> IE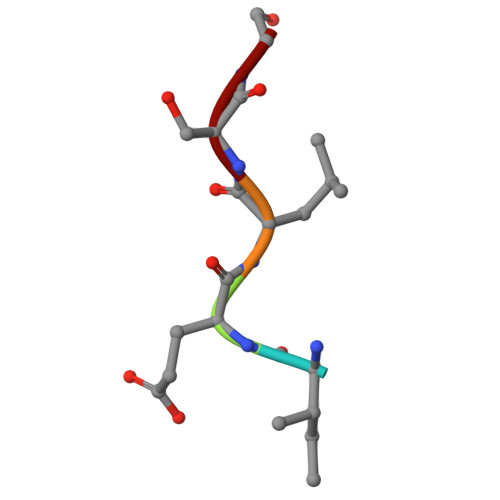LSG>MCGIVGIAGVMPVNQSIYDALTVLQHRGQDAAGIITIDANNCFRLRKANGLVSDVFEARHMQ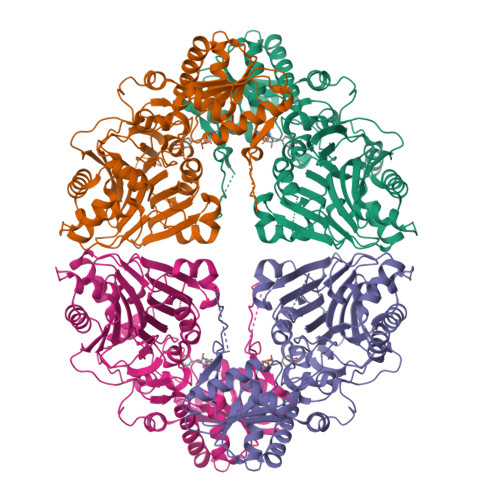RLQGNMGIGHVRYPTAGSSSASEAQPFYVNSPYGITLAHNGNLTNAHELRKKLFEEKRRHINTTSDSEILLNIFASELDNFRHYPLEADNIFAAIAATNRLIRGAYACVAMIIGHGMVAFRDPNGIRPLVLGKRDIDENRTEYMVASESVALDTLGFDFLRDVAPGEAIYITEEGQLFTRQCADNPVSNPCLFEYVYFARPDSFIDKISVYSARVNMGTKLGEKIAREWEDLDIDVVIPIPETSCDIALEIARILGKPYRQGFVKNRYVGRTFIMPGQQLRRKSVRRKLNANRAEFRDKNVLLVDDSIVRGTTSEQIIEMAREAGAKKVYLASAAPEIRFPNVYGIDMPSATELIAHGREVDEIRQIIGADGLIFQDLNDLIDAVRAENPDIQQFECSVFNGVYVTKDVDQGYLDFLDTLRNDDAKAVQRQNEVENLEMHNEGAAALEHHHHHH[4x]Peptide hormones, such as parathyroid hormone (PTH), neuropeptide Y (NPY), glucagon (GCG) and secretin (SCT), which adopt α-helical structures on binding their receptors, play key roles in human biology and are well-established biomarkers in clinical care and biomedical research. We set out to develop general methods for designing proteins that bind peptides in helical conformations. We show that by extending RFdiffusion8 to enable binder design to flexible targets, and to refining input structure models by successive noising and denoising (partial diffusion), picomolar-affinity binders can be generated to helical peptide targets by either refining designs generated with other methods, or completely de novo starting from random noise distributions without any subsequent experimental optimization. The deep learning methods largely converged on the overall solution to the helical peptide-binding design problem—groove-shaped scaffolds with helices lining the binding site—that the human designers chose in the initial Rosetta parametric approaches.

Inspired by this success at optimizing binders with RFdiffusion, we next tested its ability to design binders completely de novo through unconditional binder design. For Bim, 25/96 of the designs bound by yeast surface display, and FP on the highest-affinity design indicated a Kd of < 500 pM (bottom). Circular dichroism temperature melts indicate that both binders are stable at 95 °C. We solved the X-ray crystal structure of the Bim binder, and found that it closely matched the design model (3.0 Å resolution, 0.57 Å RMSD). A kinked helix on the binder adjacent to the interface is well recapitulated in the structure, and a cross-interface hydrogen-bond network designed between Thr73 and Asn77 of the binder and Asn20 of Bim forms in the otherwise hydrophobic interface. To our knowledge, the Bim- and PTH-binding proteins diffused starting from random noise are the highest-affinity binders to any target (protein, peptide or small molecule) achieved directly by computational design with no experimental optimization.

> MSGEEERKEKREKVRAGLKRAIAELPAEVAARCLALLDDASDEEFIEAVLEVLEAMREALVAMAREGRLDAVRRATSHINEVLVDAAELALEKGREYFRRLCLIVCDMMIELIRLEPEQTPELRRIRERLEEIRRRLEGSG;> DMRPEIWIAQELRRIGDEFNAYYARR>MDKFRVQGPTRLQGEVTISGAKNAALPILFAALLAEEPVEIQNVPKLKDIDTTMKLLTQLGTKVERDGSVWIDASNVNNFSAPYDLVKTMRASIWALGPLVARFGQGQVSLPGGDAIGARPVDLHIFGLEKLGAEIKLEEGYVKASVNGRLKGAHIVMDKVSVGATVTIMSAATLAEGTTIIENAAREPEIVDTANFLVALGAKISGQGTDRITIEGVERLGGGVYRVLPDRIETGTFLVAAAISGGKIVCRNAQPDTLDAVLAKLREAGADIETGEDWISLDMHGKRPKAVTVRTAPHPAFPTDMQAQFTLLNLVAEGTGVITETIFENRFMHVPELIR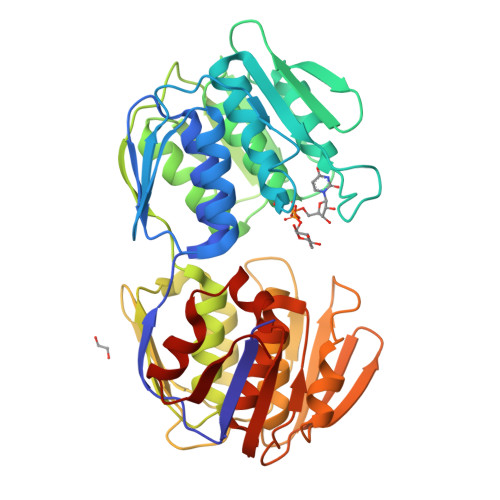MGAHAEIESNTVICHGVEKLSGAQVMATDLRASASLVLAGCIAEGTTVVDRIYHIDRGYERIEDKLRALGANIERVKGE[4x]> MGSPASDPTVFHKRYLKKIRDLGEGHFGKVSLYCYDPTNDGTGEMVAVKALKADCGPQHRSGWKQEIDILRTLYHEHIIKYKGCCEDQGEKSLQLVMEYVPLGSLRDYLPRHSIGLAQLLLFAQQICEGMAYLHSQHYIHRNLAARNVLLDNDRLVKIGDFGLAKAVPEGHEYYRVREDGDSPVFWYAPECLKEYKFYYASDV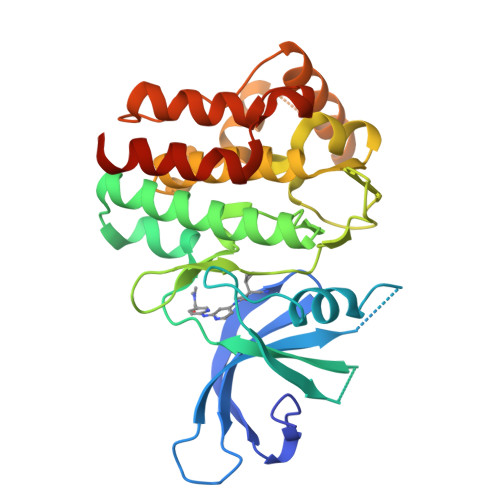WSFGVTLYELLTHCDSSQSPPTKFLELIGIAQGQMTVLRLTELLERGERLPRPDKCPCEVYHLMKNCWETEASFRPTFENLIPILKTVHEKYHHHHHH>DPFAGDPPRHPGLRVNSQKPFNAEPPAELLAERFLTPNELFFTRNHLPVPAVEPSSYRLRVDGPGGGTLSLSLAELRSRFPKHEVTATLQCAGNRRSEMSRVRPVKGLPWDIGAISTARWGGARLRDVLLHAGFPEELQGEWHVCFEGLDADPGGAPYGASIPYGRALSPAADVLLAYEMNGTELPRDHGFPVRVVVPGVVGARSVKWLRRVAVSPDESPSHWQQNDYKGFSPCVDWDTVDYRTAPAIQELPVQSAVTQPRPGAAVPPGELTVKGYAWSGGGREVVRVDVSLDGGRTWKVARLMGDKAPPGRAWAWALWE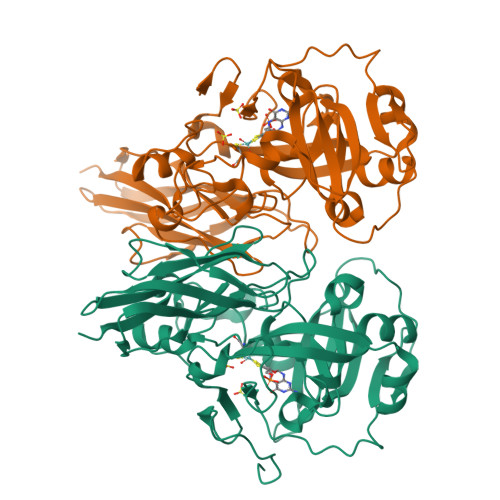LTVPVEAGTELEIVCKAVDSSYNVQPDSVAPIWNLRGVLSTAWHRVRVSVQD[2x]> MNMSGGGEQADILPANYVVKDRWKVLKKIGGGGFGEIYEAMDLLTRENVALKVESAQQPKQVLKMEVAVLKKLQGKDHVCRFIGCGRNEKFNYVVMQLQGRNLADLRRSQPRGTFTLSTTLRLGKQILESIEAIHSVGFLHRDIKPSNFAMGRLPSTYRKCYMLDFGLARQYTNTTGDVRPPRNVAGFRGTVRYASVNAHKNREMGRHDDLWSLFYMLVEFAVGQLPWRKIKDKEQVGMIKEKYEHRMLLKHMPSEFHLFLDHIASLDYFTKPDYQLIMSVFENSMKERGIAENE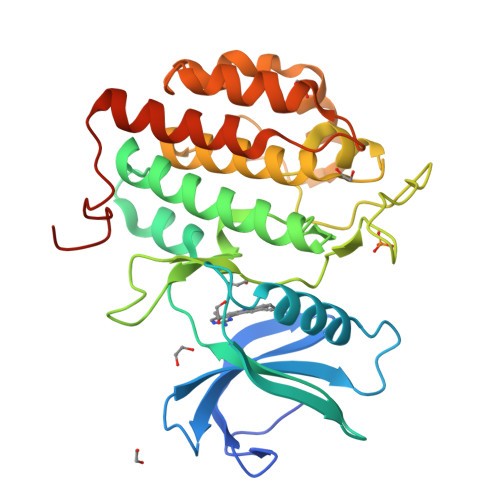AFDWEKAGTDALLS4-CARBOXYPIPERIDINE | C6 H11 N O2 | 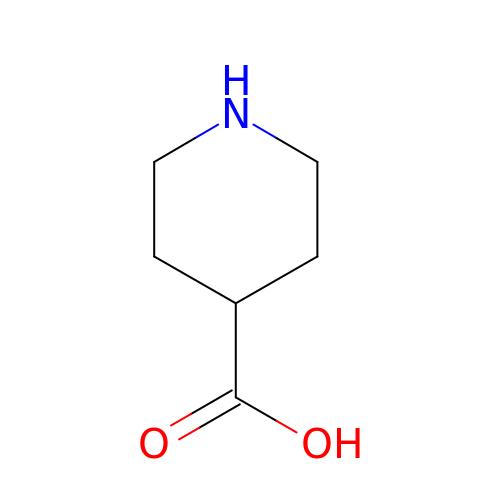SRJOCJYGOFTFLH-UHFFFAOYSA-N>GFKQDI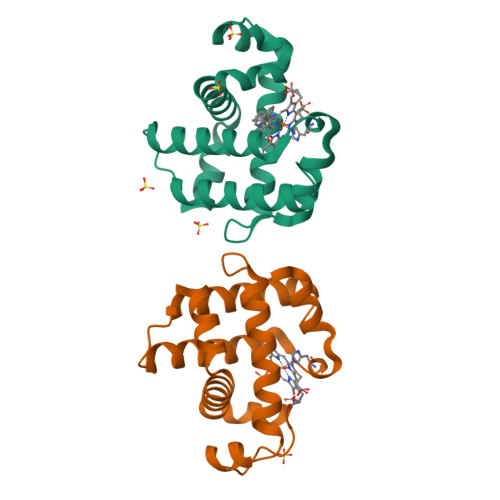ATIRGDLRTYAQDIFLAFLNKYPDERRYFKNYVGKSDQELKSMAKFGDHTEKWFNLMMEVADRATDCVPLASDANTLVQMKQHSSLTTGNFEKLFVALVEYMRASGQSFDSQSWDRFGKNLVSALSSAGMK[2x]> SNAMAMIHKFSMMGTNIVVDVNSGAVHVVDDISFDILDYYKNFTAGEIKNKLAHKYNADEIDEALREIESLEAEGLLFSEDPYKEYVSSMDRKSVVKALCLHISHDCNLRCKYCFASTGNFGGQRNMMSLEVGKKAIDFLISESGNRKNLEIDFFGGEPMMNFDVVKGIIEYARQKEKEHNKNFRFTLTTNGLLLNDENIKYINENMQNIVLSIDGRKEVNDRMRIRIDGSGCYDDILPKFKYVAESRNQDNYYVRGTFTRENMDFSNDVLHLADEGFRQISVEPVVAAK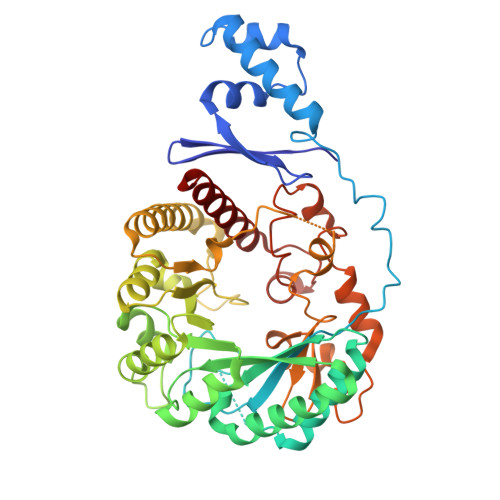DSGYDLREEDLPRLFEEYEKLAYEYVKRRKEGNWFNFFHFMIDLTQGPCIVKRLTGCGSGHEYLAVTPEGDIYPCHQFVGNEKFKMGNVKEGVLNRDIQNYFKNSNVYTKKECDSCWAKFYCSGGCAANSYNFHKDINTVYKVGCELEKKRVECALWIKAQEM> MSELERHSYDV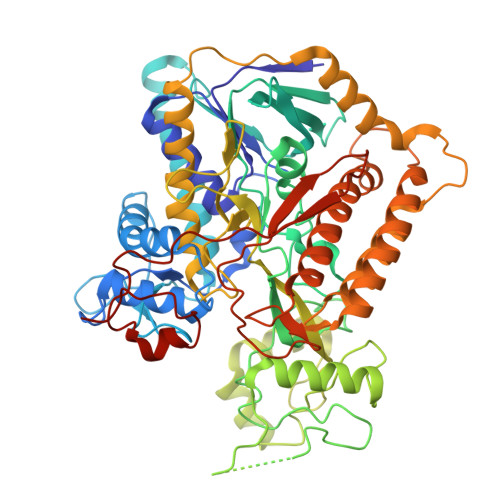VVIGAGGAGLRAVIEARERGLRVAVVTKSLFGKAHTVMAEGGCAAAMRNVNTKDSWQVHFGDTMRGGKFLNNWRMAELHAQEAPDRVWELETYGALFDRTKDGKISQRNFGGHTYPRLAHVGDRTGLEIIRTLQQKIVSLQQEDKRELGDYEARIRVFHETSITELILDDGKIAGAFGYYRETGNFVLFEAPAVVLATGGIGKSFKVSSNSWEYTGDGHALALRAGSALINMEFIQFHPTGMVWPLSVKGILVTEGVRGDGGVLKNSEGKRFMFDYIPSVFKGQYAETEEEADQWLKDNDSARRTPDLLPRDEVARAINAEVKAGRGSPHGGVYLDIASRMPAEEIKRRLPSMYHQFIELAEVDITKDAMEVGPTCHYVMGGIEVDPDTAAGATPGLFAAGECSGGMHGSNRLGGNSLSDLLVFGRRAGLGAADYVRALPDRPKVSEAAVEDATRLVLAPFEPKAEPENPYTLHAELQQSMNDLVGIIRKEAEIQEALDRLQELKRRYANVTVEGGRVFNPGWHLAIDMRNMLLVSECVAKAALQRTESRGGHTRDDYPEMDANWRNTLLVCRVSGGDPVVPDVTVTPEQQVPMRPDLLGCFELSELEKYYTPEELAEHPERKG>ADPGTS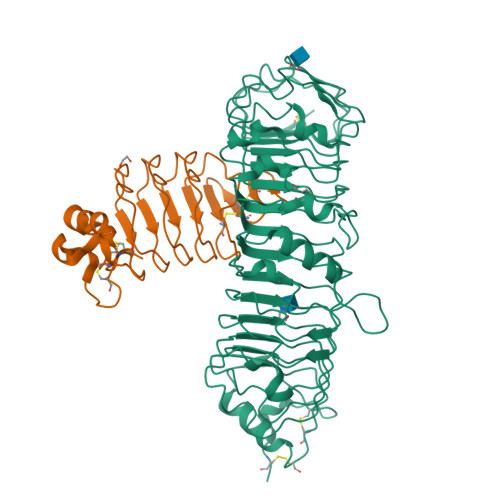ECSVIGYNAICINRGLHQVPELPAHVNYVDLSLNSIAELNETSFSRLQDLQFLKVEQQTPGLVIRNNTFRGLSSLIILKLDYNQFLQLETGAFNGLANLEVLTLTQCNLDGAVLSGNFFKPLTSLEMLVLRDNNIKKIQPASFFLNMRRFHVLDLTFNKVKSICEEDLLNFQGKHFTLLRLSSITLQDMNEYWLGWEKCGNPFKNTSITTLDLSGNGFKESMAKRFFDAIAGTKIQSLILSNSYNMGSSFGHTNFKDPDNFTFKGLEASGVKTCDLSKSKIFALLKSVFSHFTDLEQLTLAQNEINKIDDNAFWGLTHLLKLNLSQNFLGSIDSRMFENLDKLEVLDLSYNHIRALGDQSFLGLPNLKELALDTNQLKSVPDGIFDRLTSLQKIWLHTNPWDCSCPRIDYLSRWLNKNSQKEQGSAKCSGSGKPVRSIICPTSASLVPR[2x];>[2x]GGHHHHHHGSENLYFQGACPSQCSCSGTTVDCSGKSLASVPGGIPTTTQVLYLYDNQITKLEPGVFDRLVNLQQLWLEINQLTSLPAGVFDNLTQLSILNMHTNQLKSIPRGAFDNLKSLTHIWLLNNPWDCACSDILYLSGWLGQHAGKEQGQAVCSGTNTPVRAVTEASTSPSKCP> MLNRETHMKKVRKIFQKAVAGLCCISQLTAFSSIVALAETPETSPAIGKVVIKETGEGGALLGDAVFELKNNTDGTTVSQRTEAQTGEAIFSNIKPGTYTLTEAQPPVGYKPSTKQWTVEVEKNGRTTVQGEQVENREEALSDQYPQTGTYPDVQTPYQIIKVDGSEKNGQHKALNPNPYERVIPEGTLSKRIYQVNNLDDNQYGIELTVSGKTVYEQKDKSVPLDVVILLDNSNSMSNIRNKNARRAERAGEATRSLIDKITSDSENRVALVTYASTIFDGTEFTVEKGVADKNGKRLNDSLFWNYDQTSFTTNTKDYSYLKLTNDKNDIVELKNKVPTEAEDHDGNRLMYQFGATFTQKALMKADEILTQQARQNSQKVIFHITDGVPTMSYPINFNHATFAPSYQNQLNAFFSKSPNKDGILLSDFITQATSGEHTIVRGDGQSYQMFTDKTVYEKGAPAAFPVKPEKYSEMKAAGYAVIGDPINGGYIWLNWRESILAYPFNSNTAKITNHGDPTRWYYNGNIAPDGYDVFTVGIGINGDPGTDEATATSFMQSISSKPENYTNVTDTTKILEQLNRYFHTIVTEKKSIENGTITDPMGELIDLQLGTDGRFDPADYTLTANDGSRLENGQAVGGPQNDGGLLKNAKVLYDTTEKRIRVTGLYLGTDEKVTLTYNVRLNDEFVSNKFYDTNGRTTLHPKEVEQNTVRDFPIPKIRDVRKYPEITISKEKKLGDIEFIKVNKND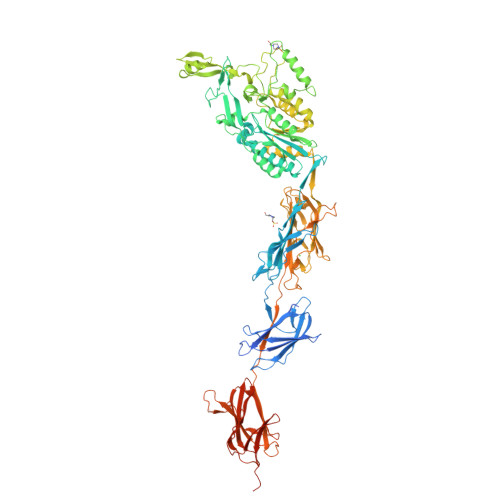KKPLRGAVFSLQKQHPDYPDIYGAIDQNGTYQNVRTGEDGKLTFKNLSDGKYRLFENSEPAGYKPVQNKPIVAFQIVNGEVRDVTSIVPQDIPAGYEFTNDKHYITNEPIPPKREYPRTGGIGMLPFYLIGCMMMGGVLLYTRKHP>[3x]XGELAQALKELAKALKEQAWALKELAQALKGX

CCs are quaternary structures comprising two or more α-helices supercoiled around each other with cyclic (Cn) or dihedral (Dn) symmetry. Here, we describe variants with all combinations of the aliphatic residues, Ile, Leu and Val, at a and d to give four classes of peptide: the ββ class, with a and d = Ile or Val; Lβ, a = Leu and d = Ile or Val; βL, a = Ile or Val and d = Leu; and LL, a = d = Leu. Peptides are named systematically appending the one-letter code for the amino acids at the a and d sites to “CC-Type2-“; e.g., CC-Hept becomes CC-Type2-LI. In summary, solution-phase data and X-ray crystal structures demonstrate conclusively that different classes of Type-2 coiled-coil (CC) peptides—i.e., based on abcdefg repeats with predominantly hydrophobic residues at a, d, e and g—adopt a range of distinct states.

Specifically, we mutated the centremost Leu at d (position 17) to Glu to give CC-Type2-IL-Sg-L17E and CC-Type2-LL-L17E. However, unlike the parents, they had accessible thermal unfolding transitions. Both transitions were pH dependent with stabilities increasing sharply below pH 6–7. We confirmed the likely involvement of Glu-17 with a pH titration of CC-Type2-LL-L17Q, which only started to unfold at pH 3.> GDGCSAGCDLALASFYVTPNQNVTNMADLFGIGAANYRSLAPYNPNIPNLDFINVGGRVNVYFTCGCRSLPGSPGATYLAGAFPFQMSRGQIYTSVAANYNNLTTAEWLQATNSYPANNIPDTAVINATVNCSCGDASISPDYGLF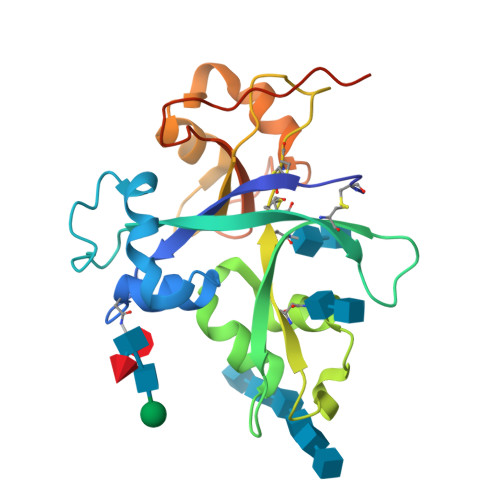LTYPLRAEDTLASVAATYGLSSQLDVVRRYNPGMESATGSGIVYIPVKDPNGSYLPLKSPGKGASHHHHHH> MWELRSIAFSRAVFAEFLATLLFVFFGLGSALNWPQALPSVLQIAMAFGLGIGTLVQALGHISGAHINPAVTVACLVGCHVSVLRAAFYVAAQLLGAVAGAALLHEITPADIRGDLAVNALSNSTTAGQAVTVELFLTLQLVLCIFASTDERRGENPGTPALSIGFSVALGHLLGIHYT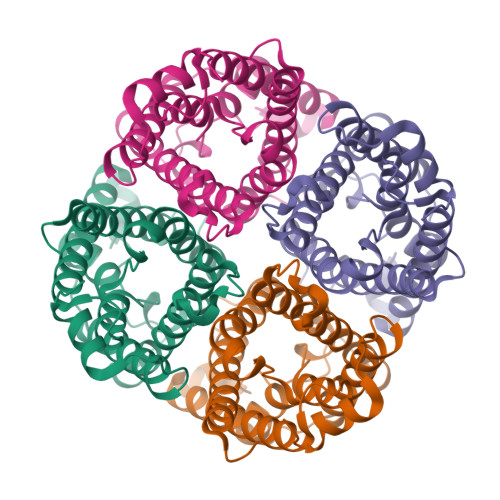GCSMNPARSLAPAVVTGKFDDHWVFWIGPLVGAILGSLLYNYVLFPPAKSLSERLAVLKGLEPDTDWEEREVRRRQSVELHSPQSLPRGTKA>[10x]MANDGY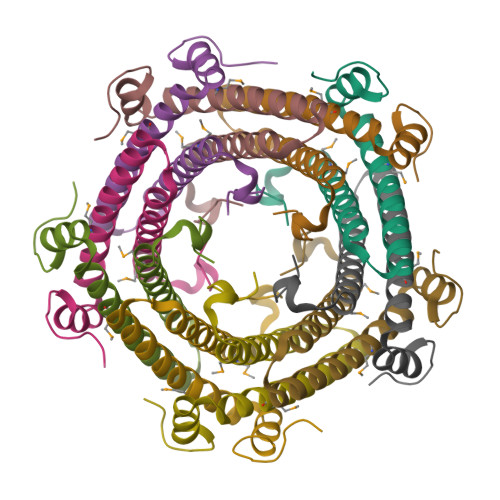FEPTQELSDETRDMHRAIISLREELEAVDLYNQRVNACKDKELKAILAHNRDEEKEHAAMLLEWIRRCDPAFDKELKDYLFTNKPIAHE> UGGAGGGAAAAGUUAUCAGGCAUGCACCUGGUAGCUAGUCUUUAAACCAAUAGAUUGCAUCGGUUUAAAAGGCAAGACCGUCAAAUUGCGGGAAAGGGGUCAACAGCCGUUCAGUACCAAGUCUCAGGGGAAACUUUGAGAUGGCCUUGCAAAGGGUAUGGUAAUAAGCUGACGGACAUGGUCCUAACCACGCAGCCAAGUCCUAAGUCAAGGAUGGUUCUUGAUAUGGAUGCAGUUCACAGACUAAAUGUCGGUCGGGGAAGAGAACCAUCCUCUUC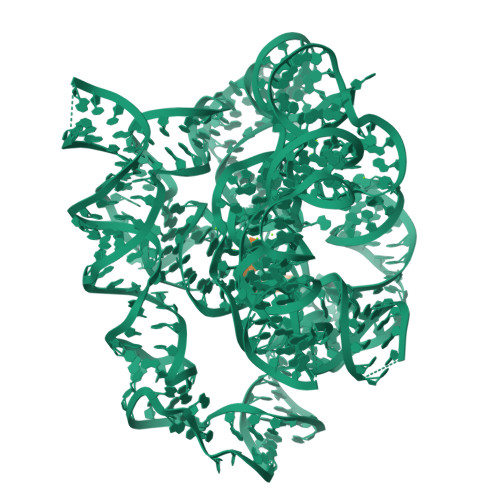UCAUAAGAUAUAGUCGGACCUCUCCUUAAUGGGAGCUAGCGGAUGAAGUGAUGCAACACUGGAGCCGCUGGGAACUAAUUUGUAUGCGAAAGUAUAUUGAUUAGUUUUGGAGUACUCG;> CUCUCTTAAGGUCC N-(4-fluorobenzoyl)-L-valyl-O-[(S)-{[(1S)-1,3-dicarboxypropyl]amino}(hydroxy)phosphoryl]-L-serine 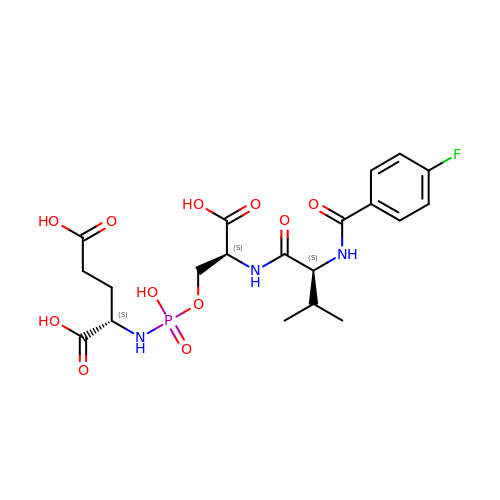| C20 H27 F N3 O11 P | OEWFGJXRSPYZTR-DZKIICNBSA-N> AAQTNAPWGLARISSTSPGTSTYYYDESAGQGSCVYVIDTGIEASHPEFEGRAQMVKTYYYSSRDGNGHGTHCAGTVGSRTYGVAKKTQLFGVKVLDDNGSGQYSTIIAGMDFVASDKNNRNCPKGVVASLSLGGGYSSSVNSAAARLQSSGVMVAVAAGNNNADARNYSPASEPSVCTVGASDRYDRRSSFSNYGSVLDIFGPGTSILSTWIGGSTRSISGTSMATP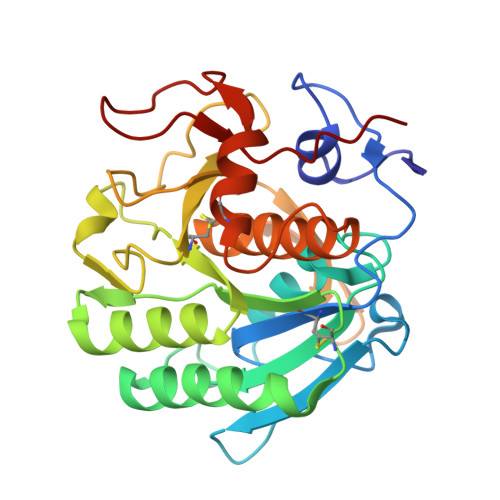HVAGLAAYLMTLGKTTAASACRYIADTANKGDLSNIPFGTVNLLAYNNYQA>[8x]MGSIGEPNRLLCFSIYVTKKPDQSE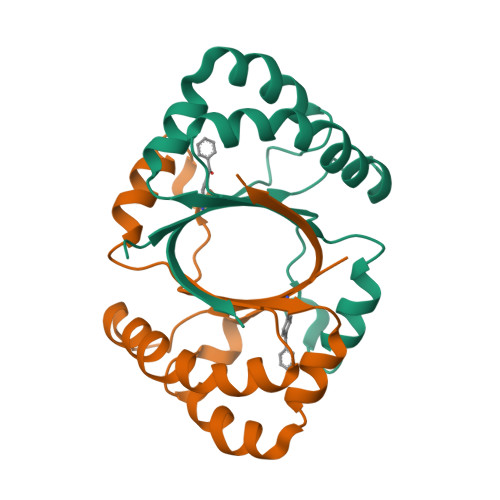EDHHNHVSKVNAPMMIPFLKKYGIVRYTVKHNDAYSKPKQAALMAGQPEENVLAYDTVFEMIVKDIESIQTMQKDEEFLRTTIPDHFNFADMTRSKGSLTWIEEFTFALEHHHHHH> MTINYQFGDVDAHGAMIRAQAGLLEAEHQAIVRDVLAAGDFWGGAGSVACQEFITQLGRNFQVI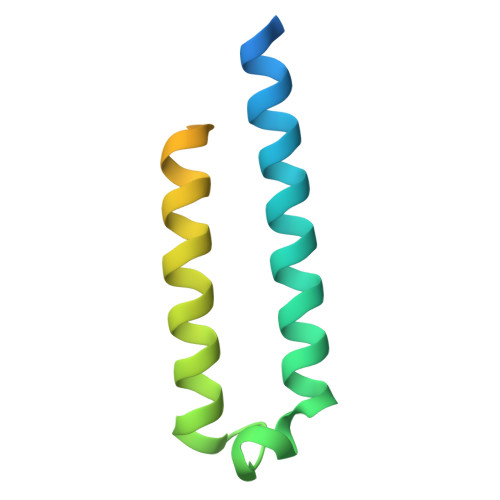YEQANAHGQKVQAAGNNMAQTDSAVGSSWATHHHHHH>[4x]MAAAAGRSLLLLLSSRGGGGGGAGGCGALTAGCFPGLGVSRHRQQQHHRTVHQRIASWQNLGAVYCSTVVPSDDVTVVYQNGLPVISVRLPSRRERCQFTLKPISDSVGVFLRQLQEEDRGIDRVAIYSPDGVRVAASTGIDLLLLDDFKLVINDLTYHVRPPKRDLLSHENAATLNDVKTLVQQLYTTLCIEQHQLNKERELIERLEDLKEQLAPLEKVRIEISRKAEKRTTLVLWGGLAYMATQFGILARLTWWE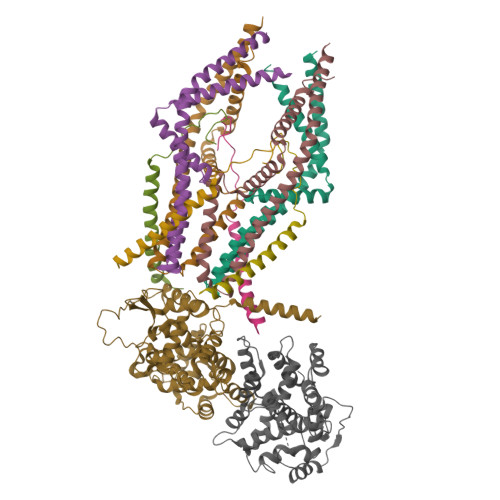YSWDIMEPVTYFITYGSAMAMYAYFVMTRQEYVYPEARDRQYLLFFHKGAKKSRFDLEKYNQLKDAIAQAEMDLKRLRDPLQVHLPLRQIGEKD;>[4x]MASGAARWLVLAPVRSGALRSGPSLRKDGDVSAAWSGSGRSLVPSRSVIVTRSGAILPKPVKMSFGLLRVFSIVIPFLYVGTLISKNFAALLEEHDIFVPEDDDDDD;> MFRLNSLSALAELAVGSRWYHGGSQPIQIRRRLMMVAFLGASAVTASTGLLWKRAHAESPPCVDNLKSDIGDKGKNKDEGDVCNHEKKTADLAPHPEEKKKKRSGFRDRKVMEYENRIRAYSTPDKIFRYFATLKVISEPGEAEVFMTPEDFVRSITPNEKQPEHLGLDQYIIKRFDGKKISQEREKFADEGSIFYTLGECGLISFSDYIFLTTVLSTPQRNFEIAFKMFDLNGDGEVDMEEFEQVQSIIRSQTSMGMRHRDRPTTGNTLKSGLCSALTTYFFGADLKGKLTIKNFLEFQRKLQHDVLKLEFERHDPVDGRITERQFGGMLLAYSGVQSKKLTAMQRQLKKHFKEGKGLTFQEVENFFTFLKNINDVDTALSFYHMAGASLDKVTMQQVARTVAKVELSDHVCDVVFALFDCDGNGELSNKEFVSIMKQRLMRGLEKPKDMGFTRLMQAMWKCAQETAWDFALPKQ;> MAAAAGSCARVAAWGGKLRRGLAVSRQAVRSPGPLAAAVAGAALAGAGAAWHHSRVSVAARDGSFTVSAQKNVEHGIIYIGKPSLRKQRFMQFSSLEHEGEYYMTPRDFLFSVMFEQMERKTSVKKLTKKDIEDTLSGIQTAGCGSTFFRDLGDKGLISYTEYLFLLTILTKPHSGFHVAFKMLDTDGNEMIEKREFFKLQKIISKQDDLMTVKTNETGYQEAIVKEPEINTTLQMRFFGKRGQRKLHYKEFRRFMENLQTEIQEMEFLQFSKGLSFMRKEDFAEWLLFFTNTENKDIYWKNVREKLSAGESISLDEFKSFCHFTTHLEDFAIAMQMFSLAHRPVRLAEFKRAVKVATGQELSNNILDTVFKIFDLDGDECLSHEEFLGVLKNRMHRGLWVPQHQSIQEYWKCVKKESIKGVKEVWKQAGKGLF> MSAPVIDKPEAGDPELPPVPEGAVMVTLKIARFNPENPDAAGWQSFRVPCLPSDRLLNLLHYVKWYLDGTLTFRRSCAHGVCGSDAMRINGVNRLACKVLMRDMLPKNPNKQLTITIEPIRGLPVEKDLVVNMEPFFDAYRAVKPFLVTSGNPPTKERIQSPTDRARYDDTTKCILCACCTTSCPVYWSEGSYFGPAAIVN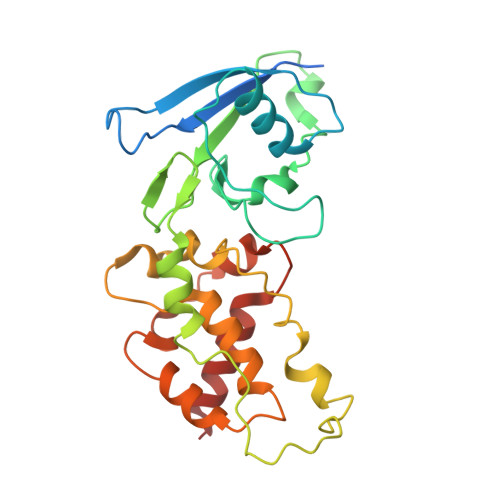AHRFIFDSRDEAAAERLDILNEVDGVWRCRTTFNCTEACPRGIQVTQAIQEVKRALMFAR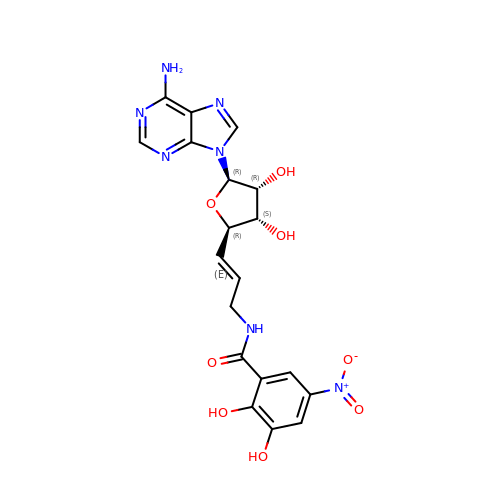N-{3-[5-(6-AMINO-PURIN-9-YL)-3,4-DIHYDROXY-TETRAHYDRO-FURAN-2-YL]-ALLYL}-2,3-DIHYDROXY-5-NITRO-BENZAMIDE | C19 H19 N7 O8 | UHHBFOLQOQSPLU-WGRQDFERSA-N As we previously demonstrated, microglia are critically dependent on CSF1R signaling for their survival, and we set out to develop specific CSF1R inhibitors that were orally bioavailable, brain-penetrant, and able to achieve robust brain-wide microglia elimination for extended periods of time. Of note, loss of function mutations in the tyrosine kinase domain of the Csf1r are associated with the development of adult-onset leukoencephalopathy with axonal spheroids and pigmented glia, the onset of which is thought to derive from microglial phenotypic alterations. To that end, we designed, synthesized, and optimized a potent, specific, orally bioavailable, and brain-penetrant CSF1R inhibitor, PLX5622, to deplete microglia for > 6 months in 5xFAD mice.

Using a structure-guided drug design strategy based on the existing CSF1R/KIT/FLT3 inhibitor PLX339710,18, combined with in vivo screening for optimal PK, brain penetrance, and microglial depletion, we created PLX5622, with crystallography revealing the interactions between PLX5622 and the CSF1R. Cell free kinase inhibitor profiling revealed that PLX5622 is highly specific for the CSF1R, showing > 20-fold selectivity over KIT and FLT3, the two most homologous receptors. Two key structural differences between PLX5622 and PLX3397 contribute to the improved selectivity based on crystallographic analysis. First, the 2-fluoro substitution on the middle pyridine ring of PLX5622 is designed to access the CSF1R-unique space next to Gly-795 (a gate-keeper to the interior allosteric pocket); both KIT and FLT3 have a bulkier cysteine at the equivalent position. Anchored on both ends by hydrogen bonds and hydrophobic packing, PLX5622 has the fluorine atom at a fixed position. As van der Waals repulsion increases in proportion to the 6th power of the distance between two atoms, a larger gate keeper residue (as seen in KIT and FLT3) will likely incur an energetic penalty for the steric hindrance. Second, the terminal pyridine group of PLX5622 is optimized to stabilize the allosteric pocket of CSF1R vacated by the displaced juxtamembrane domain.

> MKKGHHHHHHGQKPKYQVRWKIIESYEGNSYTFIDPTQLPYNEKWEFPRNNLQFGKTLGAGAFGKVVEATAFGLGKEDAVLKVAVKMLKSTAHADEKEALMSELKIMSHLGQHENIVNLLGACTHGGPVLVITEYCTYGDLLNFLRRKAEAMLGPSLSPGQDPEGLDKEDGRPLELRDLLHFSSQVAQGMAFLASKNCIHRDVAARNVLLTNGHVAKIGDFGLARDIMNDSNYIVKGNARLPVKWMAPESIFDSVYTVQSDVWSYGILLWEIFSLGLNPYPGILVNSKFYKLVKDGYQMAQPAFAPKNIYSIMQACWALEPTHRPTFQQITSFLQEQAQEDRR>MTTGLSTAGAQDIGRSSVRPYLEECTRRFQEMFDRHVVTRPTKVELTDAELREVIDDCNAAVAPLGKTVSDERWISYVGVVLWSQSPRHIKDMEAFKAVCVLNCVTFVWDDMDPALHDFGLFLPQLRKICEKYYGPEDAEVAYEAARAFVTSDHMFRDSPIKAALCTTSPEQYFRFRVTDIGVDFWMKMSYPIYRHPEFTEHAKTSLAARMTTRGLTIVNDFYSYDREVSLGQITNCFRLCDVSDETAFKEFFQARLDDMIEDIECIKAFDQLTQDVFLDLIYGNFVWTTSNK[2x]

To elucidate the dynamic interactions of TPSs with their substrates during catalysis, we investigated the bacterial diterpene synthase CotB2 as a model system. CotB2 adopts an α-helical bundle fold that is conserved among class I TPSs (PDB-ID 4OMG17). The CotB2 protein sequence exhibits a modified aspartate-rich DDXD motif12 deviating from the conventional DDXXD motif and the NSE triad NDXXSXX(R,K)(E,D) as found in bacteria and fungi, that is altered to a DTE triad in plants. Upon substrate and Mg2+ binding, TPSs undergo a discrete conformational change from an open, catalytically inactive one to a catalytically active closed conformation.

In order to biochemically confirm the importance of the entire C-terminal region for catalysis, we generated a C-terminal truncation of CotB2 terminating at R294 (CotB2ΔC). Indeed, CotB2ΔC was an inactive mutant, not capable of catalysis as shown by GC/MS. Co-crystallisation of CotB2ΔC with FGGDP resulted in the open-state conformation with no substrate bound. Additionally, this data provides further evidence that the salt-bridge between D111 and R294 is not sufficient to fully close the active site. Interestingly, there are two Mg2+-ions bound in the CotB2ΔC structure. One is fully occupied Mg2+B and the other one is partially occupied Mg2+C, which can only be fully occupied if properly coordinated by the DDXD motif upon substrate binding and the accompanying conformational changes of the active site. In combination with structural and biochemical data we could point out the importance of the properly folded C-terminus for the enzymatic activity.(2S)-2-amino-4-[hydroxy(methyl)arsoryl]butanoic acid | 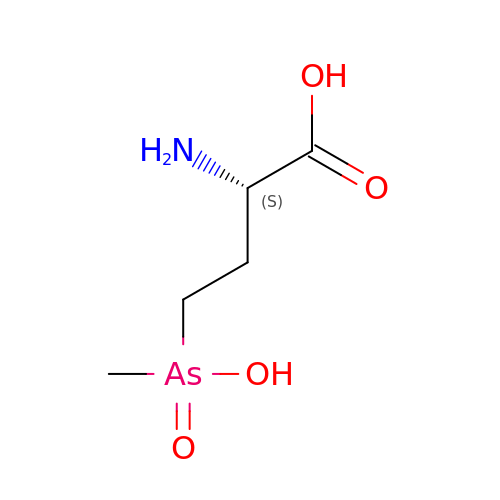C5 H12 As N O4 | CXTQPLOKUBDLTK-BYPYZUCNSA-N>GPQPLPSAPENNPEEELASKQKNEESKKRQWALEDFEIGRPLGKGKFGNVYLAREKQSKFILALKVLFKAQLEKAGVEHQLRREVEIQSHLRHPNILRLYGYFHDATRVYLILEYAPLGTVYRELQKLSKFDEQ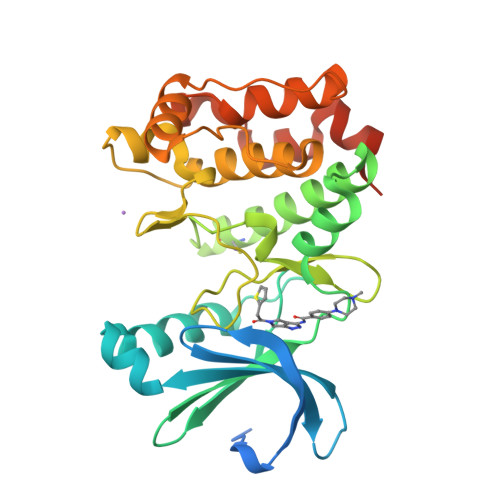RTATYITELANALSYCHSKRVIHRDIKPENLLLGSAGELKIADFGWSVHAPSSRRTTLCGTLDYLPPEMIEGRMHDEKVDLWSLGVLCYEFLVGKPPFEANTYQETYKRISRVEFTFPDFVTEGARDLISRLLKHNPSQRPMLREVLEHPWITANSSKPSNCQNKESASKQS[2x]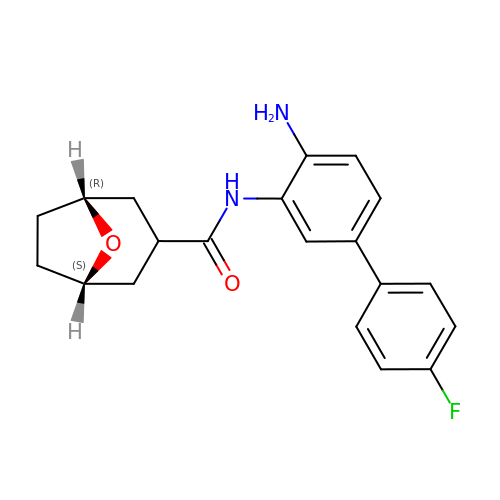(3-exo)-N-(4-amino-4'-fluoro[1,1'-biphenyl]-3-yl)-8-oxabicyclo[3.2.1]octane-3-carboxamide | C20 H21 F N2 O2 | SBKJRDAJADZOCH-XGBSXSJOSA-N>[2x]GMAKNKQEDIFDAAMQLFAERGYDGTTIPMIAEKAKVGAGTIY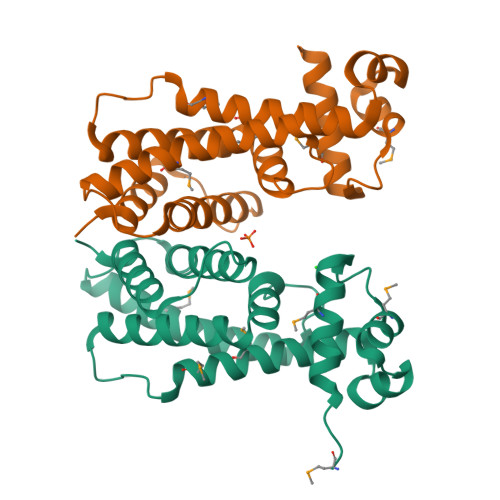RYFENKEALVNSLFSKSMLQLSEMIKTDFPVEANIREQFSHTYNRLFEFARNNVDAFLFTNSHCDSYFLDEQSKKIFDDFIGFFMNIIEDGIVKGLLRPLPPVALIIIVYQPLEKLIKVIATGQLEYSKELVKELEESSWNAIRII>[2x]MVVSENVV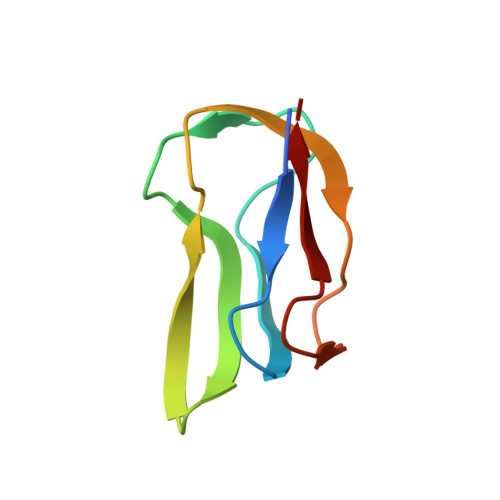SAPMPGKVLRVLVRVGDRVRVGQGLLVLEAMKMENEIPSPRDGVVKRILVKEGEAVDTGQPLIELG>[4x]MIRTGTQYLESLNDGRNVWVGNEKIDNVATHPKTRDYAQRHADFYDLHHRPDLQDVMTYIDEGGQRRAMQWFGHRDKEQLRRKRKYHETVMREMAGASFPRTPDVNNYVLTTYIDDPAPWETQSIGDDGHIKAGKIVDFIRYAREHDLNCAPQFVDPQMDRSNPDAQERSPGLRVVEKNEKGIVVNGVKAIGTGVAFADWIHIGVFFRPGIPGDQVIFAATPVNTPGVTIVCRESLVKDDKVEHPLAAQGDELDGMTVFENVFIPWSHVFHIGNPNHAKLYPQRVFDWLHYHALIRQMVRAELVAGLAVLITEHIGTNKIPAVQTRVAKLIGFHQAMLAHLIASEELGFHTPGGHYKPNILIYDFGRALYLENFSQMIYELVDLSGRSALIFASEDQWNDDKLNGWFERMNNGPVGRPHDRVKIGRVIRDLFLTDWGSRLFVFENFNGTPLQGIRMLTMQRAEFSGSGPYGKLARQVCGIDSAVTDDTEYRKTADYAKALDAARHQEEVALAGAMAI

HadA is a flavin-dependent monooxygenase catalyzing hydroxylation plus dehalogenation/denitration, which is useful for biodetoxification and biodetection. HadA belongs to the class D two-component flavin-dependent monooxygenases, which use reduced FAD (FADH–) as a substrate. The initial and committing step of the had pathway catalyzed by HadA monooxygenase is hydroxylation with removal of either halide substituents (F, Cl, Br, or I) from HPs or a nitro group (-NO2) from NP. Each protomer is composed of three domains: the N-terminal domain (residues 1–146), the β-sheet domain (residues 147–275), and the C-terminal domain (residues 276–517).

In order to gain structural and mechanistic insights into HadA, we cocrystallized the enzyme with FADH– and 4NP to obtain the first ternary structure of HadAWT−FADH–−4NP at a 2.3-Å resolution. The co-complex with FADH– and 4NP allowed identification of four binding sites for ligands in which strong electron densities could be observed for all four FADH– molecules, whereas only one 4NP molecule could be clearly seen in the expected pocket of subunit A (Inset). Of interest, two 4NP molecules were found to locate to the dimer interface between subunits C and D. The key difference between the HadAWT−FADH–−4NP structure reported here and the previously reported apo-HadAWT structure is the loop of residues 157 to 170, which assumes a distinct structure in the ternary complex, whereas it is disordered in the apo-HadAWT. The loop of residues 157 to 170 forms a lid to confine the bound FADH– via interactions with an adenosine diphosphate moiety. In the active site of HadA, the 4NP molecule binds in a hydrophobic pocket (consisting of Val155, Phe206, Phe286, Thr449, and Leu457) located between the β-sheet and C-terminal domains of each subunit. The aromatic ring of 4NP forms contacts with Phe206 face-to-face with π-π stacking and sits in van der Waals contact of Phe286, which forms π-edge interactions with Phe206. In the 4NP-binding site, a polar hydroxyl group of 4NP interacts closely with His290 (2.5 Å) on helix α9, whereas the nitro (-NO2) moiety of 4NP points toward a guanidine side chain of Arg208 (3.4 Å). We noted that, in the HadAWT complex structure, the substrate C4 position is 9 Å away from the C4a position of FADH–, which is significantly farther than the distance between the substrate hydroxylation site and the C4a-position in C2 and TtHpaB structures (5.0 and 4.9 Å, respectively). The aromatic moieties of the 4NP molecules are sandwiched with the side chains of Phe441 from subunits C and D to perfectly form face-to-face π-π-π-π or quadruple π-stacking (Phe441C = 4NP = 4NP = Phe441D) interactions. The unusual face-to-face quadruple π-stacking interactions of four aromatic moieties is the site of “dead-end” complex stabilization, which prevents the formation of C4a-hydroperoxy-FAD, causing inactivation of HadAWT.>VAQISPQYPMFTVPLPIPPVKQPRLTVTNPVNGQEIWYYEVEIKPFTHQVYPDLGSADLVGYDGMSPGPTFQVPRGVETVVRFINNAEAPNSVHLHGSFSRAAFDGWAEDITEPGSFKDYYYPNRQSARTLWYHDHAMHITAENAYRGQAGLYMLTDPAEDALNLPSGYGEFDIPMILTSKQYTANGNLVTTNGELNSFWGDVIHVNGQPWPFKNVEPRKYRFRFLDAAVSRSFGLYFADTDAIDTRLPFKVIASDSGLLEHPADTSLLYISMAERYEVVFDFSDYAGKTIELRNLGGSIGGIGTDTDYDNTDKVMRFVVADDTTQPDTSVVPANLRDVPFPSPTTNTPRQFRFGRTGPTWTINGVAFADVQNRLLANVPVGTVERWELINAGNGFTHPIHIHLVDFKVISRTSGNNARTVMPYESGLKDVVWLGRRETVVVEAHYAPFPGVYMFHCHNLIHEDHDMMAAFNATVLPDYGYNATVFVDPMEELWQARPYELGEFQAQSGQFSVQAVTERIQTMAEYRPYAAADE[2x]

Bilirubin oxidase (MvBOx; EC 1.3.3.5) from the ascomycete plant pathogen Myrothecium verrucaria (Albifimbria verrucaria) is a member of the blue multicopper oxidase family (MCO). MCOs are capable of oxidizing various organic and/or inorganic substrates and reducing oxygen to water without release of reactive oxygen species. MvBOx, composed of 534 amino acid residues, consists of three cupredoxin-like domains with four copper ions forming two active sites. T1Cu is connected with the trinuclear cluster (TNC), composed of one type II (T2Cu) and two type III (T3Cu) copper ions, via a conserved His–Cys–His motif (serving as electron transfer path).

Trp396 was mutated to alanine (MvBOxW396A) in order to enable direct solvent access to His398, to phenylalanine (MvBOxW396F) in order to introduce an aromatic residue not capable of crosslink formation, and to aspartic acid (MvBOxW396D) in order to disrupt this site by introducing negative charge. The structure of MvBOx was not affected by the mutation of Trp396 to Ala and Phe. On the structural level, the mutation of Trp396 to Phe allows for conservation of the aromatic moiety in the proximity of the T1Cu site, whereas the mutation to Ala disposes of the aromatic moiety and instead allows for solvent access to His398 coordinating T1Cu. The W396F mutant retained affinity comparable with that of the wild type, but with a lower maximal reaction velocity. The K1/2 values for the wild type and the W396F variant are comparable (0.060 ± 0.002 mM and 0.079 ± 0.004 mM, respectively) but Vmax of W396F (8.8 ± 0.5 nmol·min−1 ·μg−1) is roughly a half of the wild type value (15.8 ± 0.4 nmol·min−1 ·μg−1). ABTS binds to both mutants with a significantly lower affinity, but the maximal velocity is not affected. The presence of the Trp396–His398 adduct in MvBOx plays a minor role in its thermal stability as follows from the slight decrease of the melting temperature (Tm) of the W396A and W396F mutants (by about 5 °C and 7 °C, respectively). Mutations of Trp396 influence the enzyme activity but not the enzyme structure (except the replaced residue).>MSPFPLTSMDKAFITVLEMTPVLGTEIINYRDGMGRVLAQDVYAKDNLPPFPASVKDGYAVRAADGPGDRFIIGESQAGEQPTQTVMPGQVMRVTTGAPIPCGADAVVQVEDTELIRESDDGTEELEVRILVQARPGQDIRPIGHDIKRGECVLAKGTHMGPSEIGLLATVGVTEVEVNKFPVVAVMSTGNELLNPEDDLLPGKIRDSNRSTLLATIQEHGYPTINLGIVGDNPDDLLNALNEGISRADVIITSGGVSMGEKDYLKQVLD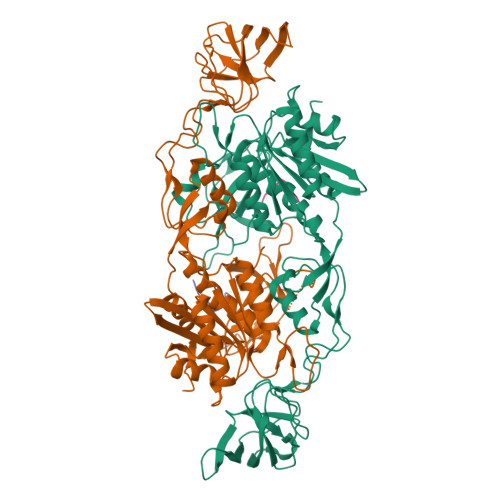IDLHAQIHFGRVFMKPGLPTTFATLDIDGVRKIIFALPGNPVSAVVTCNLFVVPALRKMQGILDPRPTIIKARLSCDVKLDPRPEYHRCILTWHHQEPLPWAQSTGNQMSSRLMSMRSANGLLMLPPKTEQYVELHKGEVVDVMVIGRL[2x];>[2x]FSIVGTLYPIN>MNGMAKKMNGARRPHGLASVLAIGTANPENCFNQDEFPDLCFRVTKSEHLTGLKEKFKRICERSTVRKRYLHLTEEILQEYPSIATYNAPSLDARQEIEVAEVPKLAARAASKAIEEWGQPKSKITHLIFCSTSGIDKPGVDCHLVHLLGLPLSVNRVMLYTLGCHAGGTVLRIAKDLAENNVGSRVLVVCTELTVMTFRGPSETDLANLIRMAIFGDGAAAVIIGADPDLSIERPIFEIYSASQTLVPNTSKAI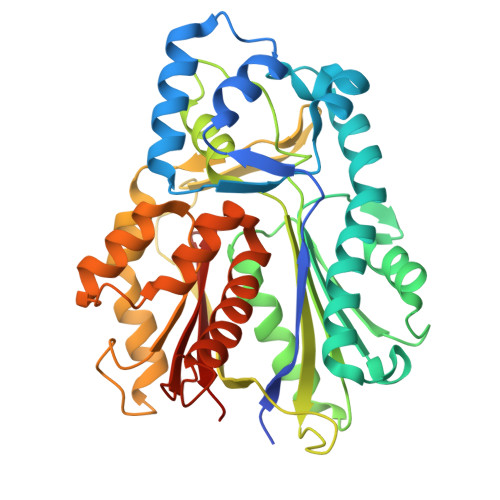HGRVLEMGLTFYVDKMVPTLVASNIEQCLDKAFSPIGIKDWNSIFWMPHPGGPAILAEIEAKLGLKPEKLRATKHVLSEYGNMSSATVLFILDEMRRRSKKEGKETTGEGLEWGVLMGFGPGVTVETVVLRAISV[4x]> GEIQWVKPNKETGRLNINGPTRTKLEPSVFHDIFEGNKEPAVLHSKDPRLEVDFEQALFSKYVGNTLHEPDEYIKEAALHYANQLKQLEINTSQMSMEEACYGTENLEAIDLHTSAGYPYSALGIKKRDILDPTTRDVSKMKFYMDKYGLDLPYSTYVKDELRSIDKIKKGKSRLIEASSLNDSVYLRMAFGHLYEAFHANPGTITGSAVGCNPDTFWSKLPILLPGSLFAFDYSGYDASLSPVWFRALELVLREIGYSEEAVSLIEGINHTHHVYRNKTYCVLGGMPSGCSGTSIFNSMINNIIIRALLIKTFKGIDLDELNMVAYGDDVLASYPFPIDCLELAKTGKEYGLTMTPADKSPCFNEVNWGNATFLKRGFLPDEQFPFLIHPTMPMREIHESIRWTKDARNTQDHVRSLCLLAWHNGKQEYEKFVSTIRSVPVGRALAIPNYENLRRNWLELFHHHHHH

The 3D (also known as 3Dpol) protein is an RNA-dependent RNA polymerase (RdRP) that plays the central role in viral RNA genome replication, and has become a major target for antiviral studies. Along with RdRPs from other RNA viruses, the polymerase catalytic core adopts an encircled right hand architecture with palm, fingers and thumb domains surrounding the active site (5–7). In summary, we identified a nucleobase-binding pocket in enterovirus RdRP by crystallography and analyzed its relevance to polymerase function through in vitro biochemical characterization and cell-based virological studies. Taken together, this pocket contributes to RdRP EC stability and virus proliferation, likely through its nucleobase binding capability.

Based on established methods in obtaining picornaviral RdRP EC crystals, we assembled a genotype-C EV71 RdRP EC using an RNA construct T31/P8 comprising a 31-nt template (T31) and an 8-nt primer (P8) to direct the incorporation of a GAGA tetra-nucleotide by providing GTP and ATP as the only NTP substrates, purified the EC by anion-exchange chromatography, and crystallized the EC. The crystal structure was solved at 1.8 Å resolution in space group C2 by molecular replacement using previously reported genotype-B EV71 RdRP EC structure as the search model. The final model had Rwork and Rfree values of 0.181 and 0.214, respectively, and the crystallographic asymmetric unit contained only one EC. The RdRP in this EC is structurally consistent with RdRPs in the previously reported enterovirus EC structures with the root-mean-square deviation (RMSD) values in the range of 0.5–1.1 Å for all superimposable α-carbon atoms (the new structure as the reference; 99–100% coverage). The majority of the RNA is well ordered including all downstream nucleotides that form a stem-loop structure. The high-resolution nature of this structure allows identification of a total of five ordered magnesium ions associated with this EC, interacting with the upstream (two ions) and downstream (two ions) RNA and residues of the catalytic motifs A and C in the palm domain (one ion). Interestingly, the guanine moiety of the 5′-end guanosine of the downstream RNA was observed to interact with a fingers domain pocket, with its guanine plane sandwiched by the imidazole moiety of the index finger residue H44 and the guanidinium moiety of the middle finger residue R277 likely through stacking interactions (average distances to the guanine plane: 3.4 Å and 3.6 Å for guanidinium and imidazole moieties, respectively; angles between neighboring planes: 10–15°). Hydrogen bonding and other hydrophobic interactions involving index finger residues N18, T21 and S45 further stabilize the guanine base, with side chains of residue S45 interacting with the guanine-specific N2 position and residue N18 interacting with the purine-specific N7 position (right).> GSHMDLLDPVDILSKMPKDFYDKLEEKKWTLRKESLEVLEKLLTDHPKLENGEYGALVSALKKVITKDSNVVLVAMAGKCLALLAKGLAKRFSNYASACVPSLLEKFKEKKPNVVTALREAIDAIYASTSLEAQQESIVESLSNKNPSVKSETALFIARALTRTQPTALNKKLLKLLTTSLVKTLNEPDPTVRDSSAEALGTLIKLMGDKAVTPLLADVDPLKMA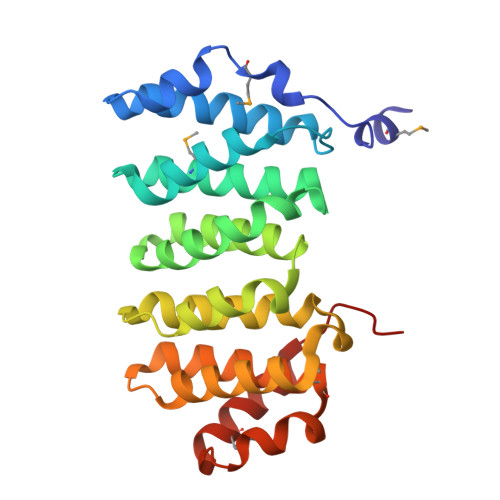KIKECQEKAEIKIKVAG Bdellovibrio bacteriovorus are small predatory bacteria which invade the periplasm of other Gram-negative bacteria, round up these (typically formerly rod-shaped) prey bacteria into spherical, osmotically stable structures called bdelloplasts, kill the prey and replicate within them. Essential to bdelloplast “sculpting” is modification, by the Bdellovibrio, of the prey cell wall peptidoglycan in the prey bacterium's periplasm. In this study we have discovered a novel use of some evolutionarily diversified class C PBPs, by the predatory bacterium Bdellovibrio bacteriovorus HD100 when they invade prey and construct the osmotically stable bdelloplast from the prey cell. Compared to the active enzyme, Bd3459 (S70A) bound significantly less Bocillin-FL as would be predicted. Together these data establish that Bd3459 is a PBP with DD-carboxy- and DD-endopeptidase activity, as suggested by the bioinformatic analysis of the protein sequence.

We solved the crystal structure of Bd3459 to 1.45 Å and this revealed predation-associated domain differences to conventional PBP4 housekeeping enzymes (loss of the regulatory domain III, alteration of domain II and a more exposed active site). Bd3459 is comprised of three domains, two of which are found in other PBP4 proteins, the classical “TP” transpeptidase domain (domain I; K38-D87 and P239-L427), and an associated domain (domain II; Y88-A238 and P428-C terminus). The largest structural difference in Bd3459 in comparison to the PBP4-grouping of enzymes is the absence from Bd3459 of a classical domain III, an all-beta structure that sits adjacent to the TP active site in conventional PBP4s and is responsible for PBP4 dimerization. Domain III has also been postulated to regulate substrate access and limit the ability of PBP4 proteins to bind bulky substrates. It is of interest (and relevance to the wide diversity of bacterial prey walls that Bdellovibrio attack) that Bd3459 possesses no compensatory regions in this part of the fold, leading to a much more accessible active site. The domain II:III:TP contacts of housekeeping PBP4 enzymes are replaced in Bd3459 by a region of novel structure, composed of AA 144–210. When building and refining the Bd3459 structure, it was apparent that a covalent modification of S70 had occurred during purification/crystallization. After being unable to crystallize the protein when HEPES/MES was excluded, we have tentatively modelled the adduct as a covalently attached HEPES molecule, with disorder distal to the C9/C10 atoms. The tetrahedral arrangement of the reacted sulphonyl group is reminiscent of a transpeptidase acylenzyme transition state, with atom O1 occupying the classical “oxyanion hole” formed by the backbone amide groups of S70 and S360. When comparing the Bd3459 and PBP4 structures, this sequence insertion takes effect between N292 and N303 and forms a “thumb-like” hairpin on the periphery of the active site pocket.

> MKVYLNSMCHMAANSKTQQIQGDDNKDDKFPLASISKVVTTLWAVDRLGPDYRFKTKLHVTPTANGSYDIHIEGSRDPLFGRNMSYFLISELNRMKITKIEKLTFDENFLLAWLAEEKPMIGGTTPKYDTVEQQASIVRATLTSSFATAISPGYYTILKTKAARIGVQMSNRPKIDVRTISFVKKAEFQKNEKSTTMVLMSAPLKTILKRMNNQSNNYIADNLYWNLGGTEAFNAYIAGKMQADTSDIEFHNGSGNNEGSVAKPVYNEATCEMMIKVLYSLDKSLSAKGYDLSDVMAVAAKDKASTVGSYGGVMAGSTTAKTGSVNKAKTLMGSVSTKNGEIYFAVLMHTDYDKSRSDWGVASQQIKNKVSQLINQNGGPKAIKYTEQLPLPFDKYSYLTKANTITTEKKLEHHHHHH>MAHHHHHHMRKIYIAGPAVFNPDMGASYYNKVRELLKKENVMPLIPTDNEATEALDIRQKNIQMIKDCDAVIADLSPFRGHEPDCGTAFEVGCAAALNKMVLTFTSDRRNMREKYGSGVDKDNLRVEGFGLPFNLMLYDGVEVFDSFESA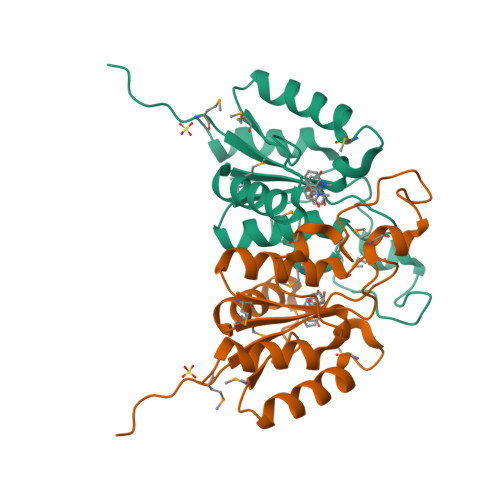FKYFLANFPSK[2x]>MNIQSTIKAVAETISTGPIPGSRKVYQAGELFPELRVPFREVAVHPSANEPPVTIYDPSGPYSDPAIQIDIEKGLPRTREALVVARGDVEEVADPRQVKPEDNGFAQGKHLAPEFPDTGRKIYRAKPGKLVTQLEYARAGIITAEMEYVAIRENLRREQDRPCVRDGEDFGASIPDFVTPEFVRQEIARGRAIIPANINHGELEPMAIGRNFLVKINANIGNSAVLSTVADEVDKLVWATRWGADTVMDLSTGRNIHNIRDWIIRNSSVPIGTVPIYQALEKVNGVAEDLNWEVFRDTLIEQCEQGVDYFTIHAGVRLPFIPMTAKRVTGIVSRGGSIMAKWCLAHHKENFLYERFDEICEIMRAYDVSFSLGDGLRPGSTADANDEAQFSELRTLGELTKVAWKHGVQVMIEGPGHVAMHKIK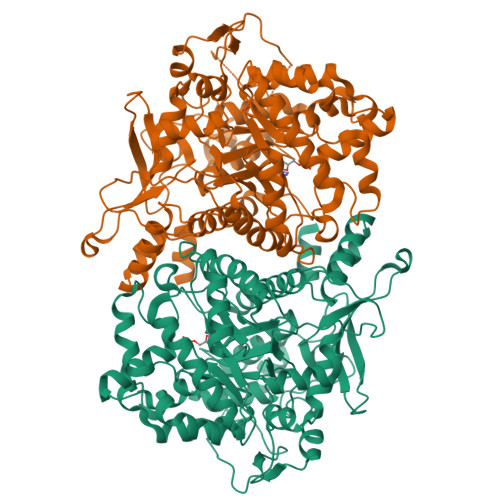ANMDEQLKHCHEAPFYTLGPLTTDIAPGYDHITSAIGAAMIGWFGTAMLCYVTPKEHLGLPDRDDVKTGVITYKLAAHAADLAKGHPGAAMWDDAISRARFEFRWEDQFNLGLDPETARKFHDETLPKEAHKTAHFCSMCGPKFCSMKISQEVRDFAAGKAPNSAELGMAEMSEKFREQGSEIYLKTE[2x]> PSSSMADFRKFFAKAKHIVIISGAGVSAESGVPTFRGAGGYWRKWQAQDLATPLAFAHNPSRVWEFYHYRREVMGSKEPNAGHRAIAECETRLGKQGRRVVVITQNIDELHRKAGTKNLLEIHGSLFKTRCTSCGVVAENYKSPICPALSGKGAPEPGTQDASIPVEKLPRCEEAGCGGLLRPHVVWFGENLDPAILEEVDRELAHCDLCLVVGTSSVV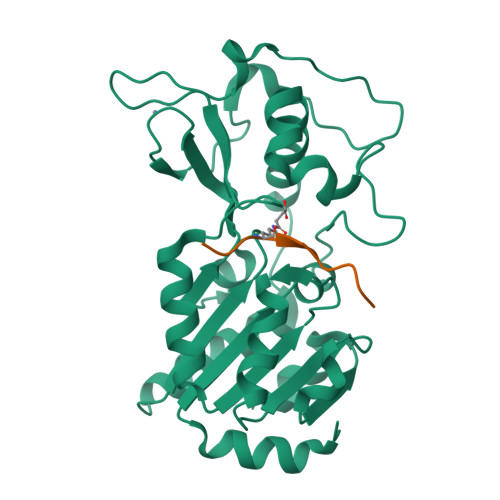YPAAMFAPQVAARGVPVAEFNTETTPATNRFRFHFQGPCGTTLPEALA;> ELNXLLGRVT>[2x]VATQPAPLYPDVGQDEAEKLGFEK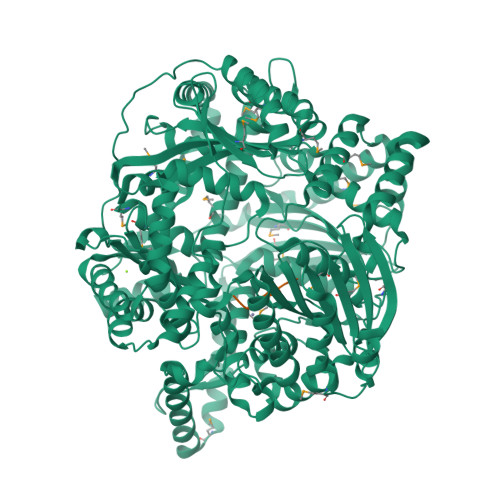VSEEFISECKSKAILFKHKKTGCEVMSVSNEDENKVFGVVFRTPPKDSTGIPHILQHSVLCGSRKYPVKEPFVELLKGSLHTFLNAFTYPDRTCYPVASTNTKDFYNLVDVYLDAVFFPKCVDDAHTFQQEGWHYELNDPSEDISYKGVVFNEMKGVYSQPDNILGRIAQQALSPENTYGVDSGGDPKDIPNLTFEEFKEFHRQYYHPSNARIWFYGDDDPVHRLRVLSEYLDMFEASPSPNSSKIKFQKLFSEPVRLVEKYPAGRDGDLKKKHMLCVNWLLSEKPLDLQTQLALGFLDHLMLGTPASPLRKILLESGLGEALVSSGLSDELLQPQFGIGLKGVSEENVQKVEELIMDTLKKLAEEGFDNDAVEASMNTIEFSLRENNTGSFPRGLSLMLQSISKWIYDMDPFEPLKYTEPLKALKTRIAEEGSKAVFSPLIEKLILNNSHRVTIEMQPDPEKATQEEVEEKNILEKVKAAMTEEDLAELARATEELKLKQETPDPPEALRCVPSLNLGDIPKEPTYVPTEVGDINGVKVLRHDLFTNDIIYTEVVFDIGSLKHELLPLVPLFCQSLLEMGTKDLTFVQLNQLIGRKTGGISVYPLTSSVRGKDEPCSKIIVRGKSMAGRADDLFNLMNCLLQEVQFTDQQRFKQFVSQSRARMENRLRGSGHGIAAARMDAMLNIAGWMSEQMGGLSYLEFLHTLEKKVDEDWEGISSSLEEIRRSLLARNGCIVNMTADGKSLTNVEKSVAKFLDLLPENPSGGLVTWDGRLPLRNEAIVIPTQVNYVGKAGNIYSTGYELDGSAYVISKHISNTWLWDRVRVSGGAYGGFCDFDSHSGVFSYLSYRDPNLLKTLDIYDGTGDFLRGLDVDQETLTKAIIGTIGDVDSYQLPDAKGYSSLLRHLLGVTDEERQRKREEILTTSLKDFKDFAQAIDVVRDKGVAVAVASAEDIDAANNERSNFFEVKKAL;>[2x]AALTRA>[2x]MMEYKIVENGLTYRIGNGASVPISNTGELIKGLRNYGPYEVPSLKYNQIALIHNNQFSSLINQLKSQISSKIDEVWHIHNINISEFIYDSPHFDSIKSQVDNAIDTGVDGIMLVLPEYNTPLYYKLKSYLINSIPSQFMRYDILSNRNLTFYVDNLLVQFVSKLGGKPWILNVDPEKGSDIIIGTGATRIDNVNLFCFAMVFKKDGTMLWNEISPIVTSSEYLTYLKSTIKKVVYGFKKSNPDWDVEKLTLHVSGKRPKMKDGETKILKETVEELKKQEMVSRDVKYAILHLNETHPFWVMGDPNNRFHPYEGTKVKLSSKRYLLTLLQPYLKRNGLEMVTPIKPLSVEIVSDNWTSEEYYHNVHEILDEIYYLSKMNWRGFRSRNLPVTVNYPKLVAGIIANVNRYGGYPINPEGNRSLQTNPWFL

AfPiwi is a model PIWI/MID domain protein, corresponding to the “PIWI lobe” of a full-length Argonaute protein (Parker et al., 2004; Song et al., 2004; Yuan et al., 2005). Crystal structures show that the seed region of the guide strand is anchored via its phosphodiester backbone to the PIWI/MID domain of Argonaute and that this complex provides the platform for target mRNA recognition (Ma et al., 2005; Parker et al., 2005; Wang et al., 2008). We show, using isothermal titration calorimetry (ITC), that association with a PIWI/MID domain protein (AfPiwi from Archaeoglobus fulgidus) greatly enhances the affinity of the seed-target interaction. Thus, association of the guide strand with the PIWI/MID domain generates an enhanced affinity anchor site over the seed that can promote fidelity in target recognition and stabilize and guide the assembly of the active silencing complex.

Some of our experiments were performed using DNA mimics of the guide and target strands, so we first determined the structure of AfPiwi in complex with DNA mimics of guide and target strands, and compared the structure to a similar complex with RNA. The structure was determined by molecular replacement to a resolution of 1.9 Å. The structure superimposes closely with the RNA complex (Parker et al., 2005; Ma et al., 2005), with the guide strand anchored to AfPiwi via its 5′ phosphate group and the phosphodiester backbone of the seed region. At the 5′ end, the nucleic acid duplex is distorted such that the G1 and T1 bases are unwound with G1 being displaced into the conserved 5′ binding pocket. The target strand interacts primarily with the base edges of the guide. The principal differences are the formation of B-form duplex rather than A-form duplex and the insertion of the DNA T1 target nucleotide into a pocket in AfPiwi, forming interactions with Ile30, Phe151, and Asp154. In contrast, in the RNA complex, the T1 nucleotide is significantly distorted and exposed entirely to solvent, indicating that the RNA nucleotide is incompatible with the binding pocket. The interactions between conserved residues in AfPiwi and the phosphodiester backbone of the seed region of the guide are identical or similar in most cases to those in the RNA complex. AfPiwi binds DNA more tightly than RNA (Ma et al., 2005). Furthermore, the crystal structures of the AfPiwi RNA/RNA and DNA/DNA complexes show that in both cases target nucleotides T2 to T8 make no contacts to the protein, interacting with the complex through base pairing to the guide only.>[2x]GFARLKRSLLKTKENLGSGFISLFRGKKIDDDLFEELEEQLLIADVGVETTRKIITNLTEGAS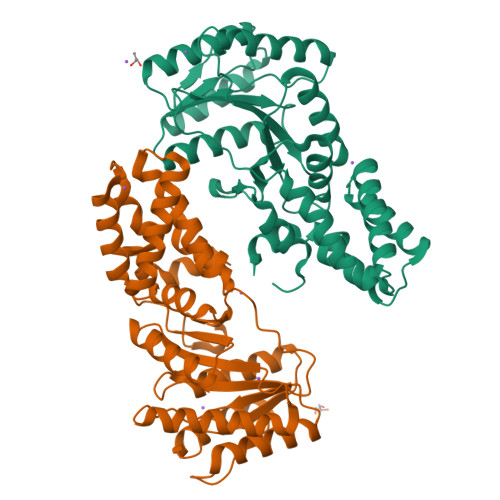RKQLRDAEALYGLLKEEMGEILAKVDEPLNVEGKAPFVILMVGVNGVGKTTTIGKLARQFEQQGKSVMLAAGDTFRAAAVEQLQVWGQRNNIPVIAQHTGADSASVIFDAIQAAKARNIDVLIADTAGRLQNKSHLMEELKKIVRVMKKLDVEAPHEVMLTIDASTGQNAVSQAKLFHEAVGLTGITLTKLDGTAKGGVIFSVADQFGIPIRYIGVGERIEDLRPFKADDFIEALFARED SINEFUNGIN | C15 H23 N7 O5 | 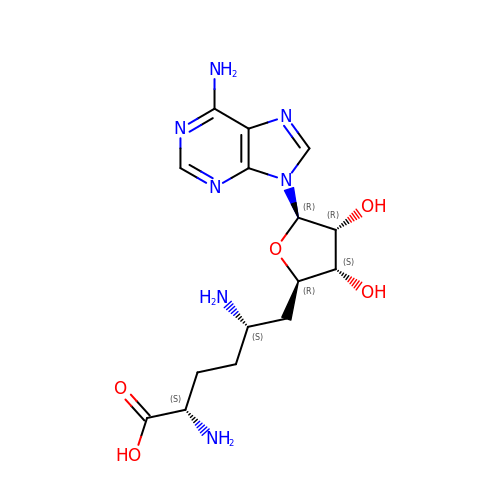LMXOHSDXUQEUSF-YECHIGJVSA-N Halohydrin dehalogenases (HHDHs; also, haloalcohol dehalogenases or epoxidases, halohydrin hydrogen-halide-lyases) are biotechnologically relevant enzymes for the production of chiral epoxides and β-substituted alcohols. In their natural function, they catalyze the reversible dehalogenation of vicinal haloalcohols with formation of the corresponding epoxides. HHDHs possess a catalytic triad composed of serine, tyrosine and arginine. Protein engineering of halohydrin dehalogenase HheG for thermostabilization revealed several residues with positive impact on the apparent melting temperature.

After solving and inspecting all of these crystal forms, two (T123G_1 and T123G_2) were chosen for final refinement and analysis, since they encompassed all structural changes with respect to the structure of the wild-type protein. More significantly, the flexible loop connecting strand β2 and helix α2 (residues 39 to 47) adopts a different conformation in three out of eight chains in the asymmetric unit of crystal form T123G_2. As a consequence, the loop moves towards residue 123 and leads to a partial covering of the active site cleft, resulting in significantly restricted access to the active site. It must be noted that this different loop conformation is enforced by altered contacts in this crystal form as the position of the loop in its open conformation is occupied by crystallographic neighbors. However, to form a crystal in which the closed loop conformation is observable, this conformation has to be present during crystallization. Therefore, the T123G mutant favors the closed state more than the wild-type enzyme. In variant T123G, on the other hand, the additional space generated by the missing side chain is partially occupied by L103, resulting in a slight displacement of a loop connecting strand β4 and helix α4 (residues 101 to 107) that covers the catalytic triad. The most obvious change in loop position can be seen in variant T123G, where the loop is moved significantly toward residue 123, partially closing the active site cleft. Therefore, even though HheG wild-type and variant T123G display similar RMSF values, the average loop positions are very distinct. This partially closed conformation for T123G is in line with the observed loop conformation of some chains of the asymmetric unit of the T123G_2 crystal form described in the previous section. Variant T123G was the most active one with a 5-fold higher initial reaction velocity in the azidolysis of cyclohexene oxide compared to wild-type HheG.

>[8x]ENRPVALITMATGYVGPALARTMADRGFDLVLHGTAGDGTMVGVEESFDSQIADLAKRGADVLTISDVDLTTRTGNQSMIERVLERFGRLDSACLVTGLIVTGKFLDMTDDQWAKVKAGNLDMVFHGLQAVLPPMVAAGAGQCVVFTSATGGRPDPMVSIYGGTRAGANGIVRAVGLEHARHGVQVNAIGTNYMDFPGFLKASRADGDPERRAMIEAQVPLRRLGTMDELSSVTAGLLDGSNRFQTGQFFDFSGGWGA propadienyl 6-deoxy-alpha-L-galactopyranoside | C9 H14 O5 | 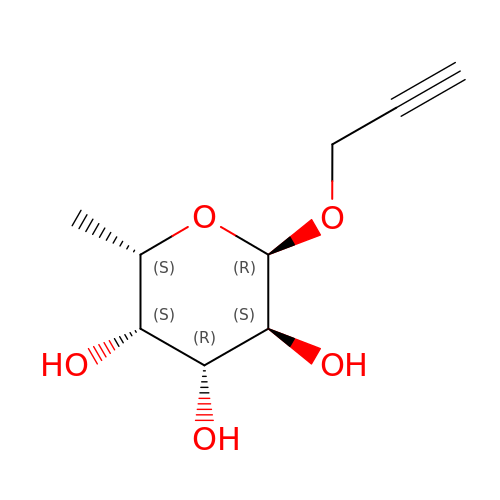BVZDJWONINIPAQ-JTPBWFLFSA-N> KEALEIEKNSRKPPPYKHIKANKVIGKVQIQVADLSEIPRCNCKPADENPCGLESECLNRMLQYECHPQVCPAGDRCQNQCFTKRLYPDAEIIKTERRGWGLRTKRSIKKGEFVNEYVGELIDEEECRLRIKRAHENSVTNFYMLTVTKDRIIDAGPKGNYSRFMNHSCNPNCETQKWTVNGDVRVGLFALCDIPAGMELTFNYNLDCLGNGRTECHCGADNCSGFLG

Protein methyltransferases are enzymes that add covalent methyl groups to arginine or lysine side chains of proteins employing S-adenosyl-L-methionine (SAM) as a cofactor. The NSD family members are large, multi-domain enzymes that, in addition to the catalytic SET (Su(var), E(z) and Trithorax) domain, include known epigenetic reader domains such as PHD and PWWP domains, and these reader domains likely contribute to chromatin binding. Given the evidence linking NSD family members and oncology, there is great interest in developing potent and selective inhibitors for one or more members of the NSD family.

Two peptides were synthesized based on the H4K44 substrate sequence used in the assay, PTD1 (15 residues) and PTD2 (5 residues), where K44 has been replaced with Nle. In order to understand the binding mode of the peptide to the protein and to further validate these inhibitors, the structure of PTD2 was solved with a SET domain construct of WHSC1L1 comprising amino acids 1054–1285. WHSC1 and WHSC1L1 are highly homologous proteins with 45% identity (53% similarity) overall and are 78% identical (84% similar) in the sequence corresponding to the construct utilized for structure determination. The 1.61 Å ternary structure of WHSC1L1 1054–1285 with PTD2 and SAM confirms the inhibitor peptide binds in the histone binding pocket with the norleucine residue occupying the substrate lysine channel. Significant reorganization of the autoinhibitory loop is required for peptide binding, as the peptide overlaps with the loop in both the WHSC1 and NSD1 structures, both of which are in autoinhibitory conformations. In the complexed structure, the autoinhibitory loop moves towards the C-terminus of the construct to open the binding site for the peptide. The interactions of the peptide with the protein are dominated by hydrogen bonds; with the exception of the N-terminal acetyl group and NH of the glycine residue, all backbone amide and carbonyl moieties are involved in hydrogen bonds. Met 1201 and Thr 1203 of the autoinhibitory loop, Thr 1323 and residues 1260–1264 make direct and/or water mediated interactions with peptide. As previously noted, the norleucine residue points towards SAM and the terminal methyl of the unnatural amino acid is 4.1 Å from the SAM methyl group. The alkyl chain also makes hydrophobic interactions with Tyr 1262 and Phe 1259.>MTTAPQEPPARPLQAGSGAGPAPGRAMRSTTLLALLALVLLYLVSGALVFRALEQPHEQQAQRELGEVREKFLRAHPCVSDQELGLLIKEVADALG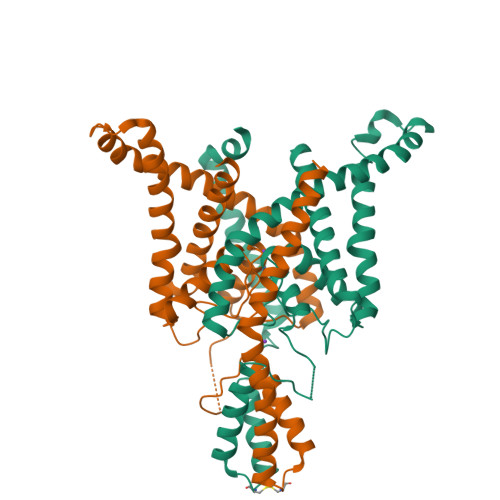GGADPETQSTSQSSHSAWDLGSAFFFSGTIITTIGYGNVALRTDAGRLFCIFYALVGIPLFGILLAGVGDRLGSSLRHGIGHIEAIFLKWHVPPELVRVLSAMLFLLIGCLLFVLTPTFVFCYMEDWSKLEAIYFVIVTLTTVGFGDYVAGADPRQDSPAYQPLVSFWILLGLAYFASVLTTIGNWLRVVSRRTRAEMGGLTAQSNSLEVLFQ[2x]> MASISEVIRVSLQQEGRAIAPDNMNAVGIITGNQGVLSTADRYRIYRTAAAVASDFGASSQESAFANTFFDTTPNPISAGGVLVIGYWRSASETVAATSATLVSEQTSESVLIPLLNAINDGSFTITVDGGTEQEVTALDFTGVSELSEVATILNSAITGATVSEDNGYFKVTSSTTGATSLLSYL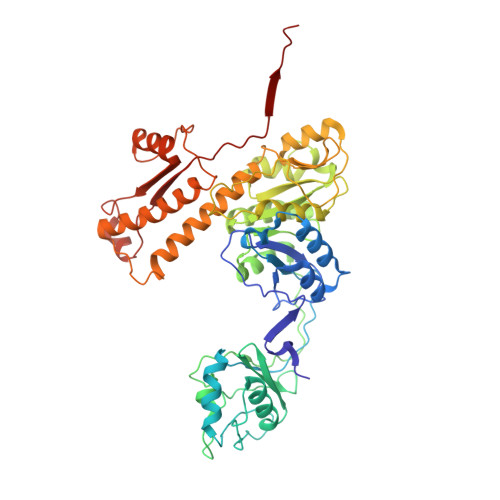GVATSGTDISAVLGMNSESGAVLTQGTDQVVLPAETKLEGITAIKSEVNIKGAMFIDQILDADIPGIASFAGANNMLVYEVFDTGYLSKNVSNPVWAVKLAGQSNFRCLLSKSGNRKFAATYMARMHTVLFSGQNTAITMQLKELSVTAEEYTDTEIANAKTVGLDLLTTIKNEQALLTSGANDFCDNVYNLEAFRDEIQTNNYNLLKTTSTKIPQTDPGMDTIEDDTEKTCEKYVRNGVFAPGTWTRSDFFGDRQQFVDAIAQKGYYVLIGDLADQTTAERQSRVSPVIQIAVKNAGAVHEEDIIISVNL> TRATNDERCKILEQRLEQGM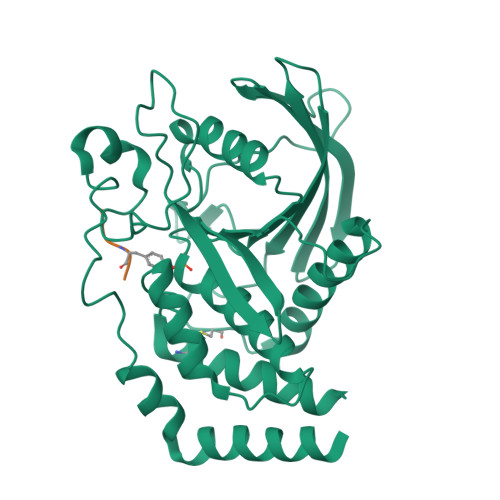VFTEYERILKKRLVDGECSTARLPENAERNRFQDVLPYDDVRVELVPTKENNTGYINASHIKVSVSGIEWDYIATQGPLQNTCQDFWQMVWEQGIAIIAMVTAEEEGGREKSFRYWPRLGSRHNTVTYGRFKITTRFRTDSGCYATTGLKMKHLLTGQERTVWHLQYTDWPEHGCPEDLKGFLSYLEEIQSVRRHTNSTSDPQSPNPPLLVHSSAGVGRTGVVILSEIMIACLEHNEVLDIPRVLDMLRQQRMMLVQTLCQYTFVYRVLIQFLKSSRLI;> EPQYQ4-(beta-D-glucopyranosyloxy)-2,2-dihydroxybutyl 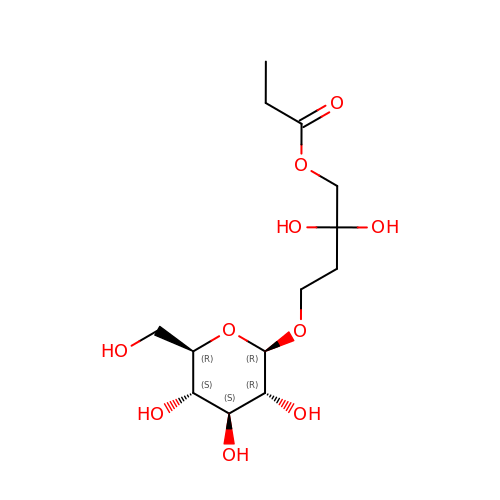propanoate | C13 H24 O10 | LNJDDDXXDSOXEJ-DVYMNCLGSA-N>[2x]MFENITAAPADPILGLADLFRADERPGKINLGIGVYKDETGKTPVLTSVKKAEQYLLENETTKNYLGIDGIPEFGRCTQELLFGKGSALINDKRARTAQTPGGTGALRVAADFLAKNTSVKRVWVSNPSHPNHKSVFNSAGLEVREYAYYDAENHTLDFDALINSLNEAQAGDVVLFHGCCHNPTGIDPTLEQWQTLAQLSVEKGWLP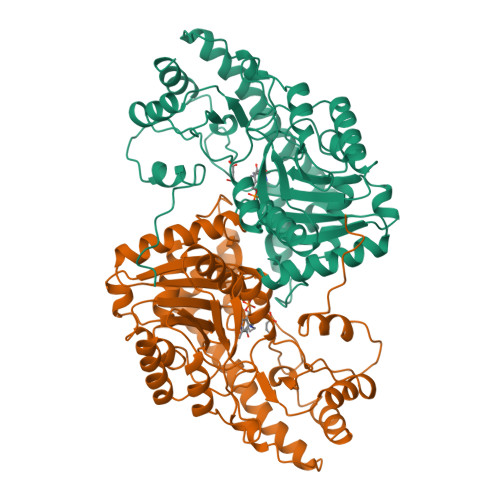LFDFAYQGFARGLEEDAEGLRAFAAMHKELIVASSYSKNFGLYNERVGACTLVAADSETVDRAFSQMKAAIRANYSNPPAHGASVVATILSNDALRAIWEQELTDMRQRIQRMRQLFVNTLQEKGANRDFSFIIKQNGMFSFSGLTKEQVLRLREEFGVYAVASGRVNVAGMTPDNMAPLCEAIVAVL> GSVFPSSVYVPDEWEVSREKITLLRELGQGSFGMVYEGNARDIIKGEAETRVAVKTVNESASLRERIEFLNEASVMKGFTCHHVVRLLGVVSKGQPTLVVMELMAHGDLKSYLRSLRPEAENNPGRPPPTLQEMIQMAAEIADGMAYLNAKKFVHRNLAARNCMVAHDFTVKIGDFGMTRDIYETDYYRKGGKGLLPVRWMAPESLKDGVFTTSSDMWSFGVVLWEITSLAEQPYQGLSNEQVLKFVMDGGYLDQPDNCPERVTDLMRMCWQFNPKMRPTFLEIVNLLKDDLHPSFPEVSFFH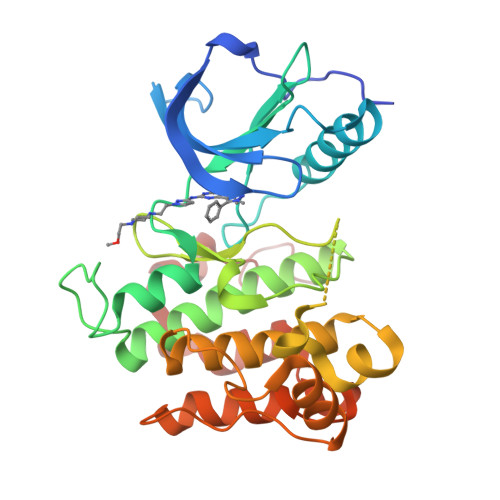SEENK> WYHRIDHTVLLGALP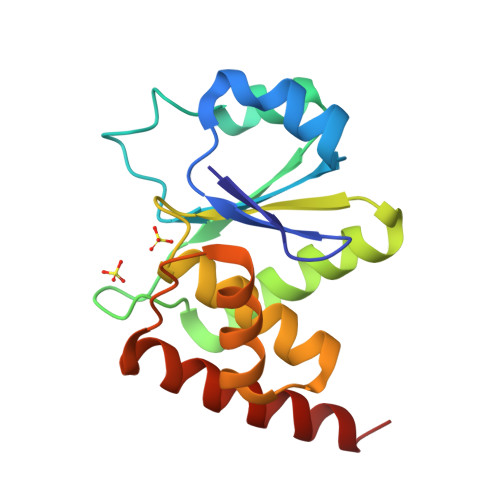LKNMTRRLVLDENVRGVITMNEEYETRFLCNTSKEWKKAGVEQLRLSTVDMTGVPTLANLHKGVQFALKYQALGQCVYVHCKAGRSRSATMVAAYLIQVHNWSPEEAIEAIAKIRSHISIRPSQLEVLKEFHKEITARAAKN> ADPGAPTPVNPCCYYPCQHQGICVRFGLDRYQCDCTRTGYSGPNCTIPGLWTWLRNSLRPSPSFTHFLLTHGRWFWEFVNATFIREMLMRLVLTVRSNLIPSPPTYNSAHDYISWESFSNVSYYTRILPSVPKDCPTPMGTKGKKQLPDAQLLARRFLLRRKFIPDPQGTNLMFAFFAQHFTHQFFKTSGKMGPGFTKALGHGVDLGHIYGDNLERQYQLRLFKDGKLKYQVLDGEMYPPSVEEAPVLMHYPRGIPPQSQMAVGQEVFGLLPGLMLYATLWLREHNRVCDLLKAEHPTWGDEQLFQTTRLILIGETIKIVIEEYVQQLSGYFLQLKFDPELLFGVQFQYRNRIAMEFNHLYHWHPLMPDSFKVGSQEYSYEQFLFNTSMLVDYGVEALVDAFSRQIAGRIGGGRNMDHHILHVAVDVIRESREMRLQPFNEYRKRFGMKPYTSFQELVGEKEMAAELEELYGDIDALEFYPGLLLEKCHPNSIFGESMIEIGAPFSLKGLLGNPICSPEYWKPSTFGGEVGFNIVKTATLKKLVCLNTKTCPYVSFRVPDASQDDGPAVERPSTEL

Prostaglandin endoperoxide H synthases (PGHSs), also known as cyclooxygenases (COXs), catalyze the conversion of free arachidonic acid (AA), released from cell membrane upon mitogen or mechanical stimuli, into Prostaglandin H2 (PGH2), that represents the committed step in the biosynthesis of prostaglandins, prostacyclin, and thromboxane. The known COX isoforms (COX-1 and COX-2) are the product of two different genes. In contrast to COX-1, COX-2 expression is typically inducible in response to pro-inflammatory events and growth factors. COX-1 is a functional dimer, and dimerization is strictly required for structural integrity and activity.

In this paper, we report the first three-dimensional crystal structure of hCOX-1 along with an extensive structural comparison with known crystal structures of the constitutive (COX-1) and inducible (COX-2) isoforms of the prostaglandin-endoperoxide H synthase. hCOX-1 has a very high sequence identity with oCOX-1 (92%) and, like the ovine enzyme, also crystallizes in a hexagonal space group in the presence of lithium chloride and sodium citrate. The hCOX-1 crystal shows P 6522 symmetry, and its asymmetric unit contains a single protein molecule. According to the PISA server, the protein in the asymmetric unit interacts with a symmetry-related molecule (symmetry operation y, x, − z-1/3) to form a dimeric biological unit, whose interaction interface is about 26% of the solvent-exposed area of the monomer. The high free energy calculated for dimer dissociation (17.6 kcal/M) suggests that such a biological unit is thermodynamically stable. Diffraction data quality is enough to model the expected N-acetyl glucosamine (NAG) chain on N68, N410, N144 that are shown in stick representation in Fig. 2a. To make sure that such electron density features related to the heme molecule are not an artifact due to an incorrect choice of space group, data were reprocessed in the alternative space group P 65, suggested by the indexing process, where the two protein chains can have different conformations, but no difference was observed. Unable to confirm the presence of the heme in our crystal structure, we decided not to include such a prosthetic group in the final model. In the case of pairwise comparison between oCOX-1 structures and our hCOX-1, the average of the RMSD values is ~ 0.5 Å, and it is ~ 0.8 Å in the case of comparison with hCOX-2 crystal structures, despite the low sequence identity (60%). We delineated two regions characterized by positional deviations between hCOX-1 and all the other structures investigated: the α6-α7 loop, comprising residues from 270 to 290, and the region 70–110, covering the first two α-helices of the membrane-binding domain. On the contrary, inter-molecular hydrogen bonds do not involve glycosylation sites in hCOX-1, differently from oCOX-1 and hCOX-2.>[2x]GHMEIDPKDLTFLKELGTGQFGVVKYGKWRGQYDVAIKMIKEGSMSEDEFIEEAKVMMNLSHEKLVQLYGVCTKQRPIFIITEYMANGCLLNYLREMRHRFQTQQLLEMCKDVCEAMEYLESKQFLHRDLAARNCLVNDQGVVKVSDFGLSRYVLDDEYTSSVGSKFPVRWSPPEVLMYSKFSSKSD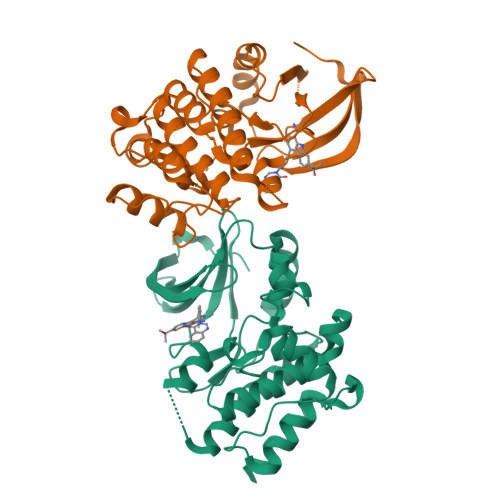IWAFGVLMWEIYSLGKMPYERFTNSETAEHIAQGLRLYRPHLASEKVYTIMYSCWHEKADERPTFKILLSNILDVMDEES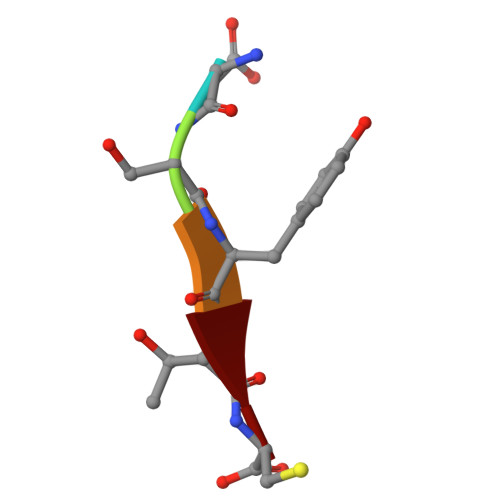> DSYTC> PISPIETVPVKLKPGMDGPKVKQWPLTEEKIKALVEICTEMEKEGKISKIGPENPYNTPVFAIKKKDSTKWRKLVDFRELNKRTQD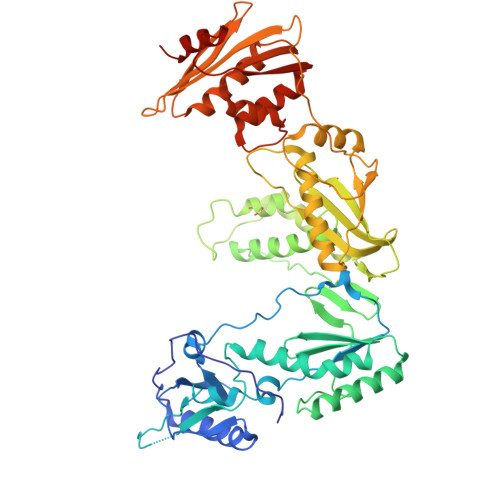FWEVQLGIPHPAGLKKKKSVTILDVGDAYFSVPLDEDFRKYTAFTIPSINNETPGIRYQYNVLPQGWKGSPAIFQSSMTKILEPFRKQNPDIVIYQYMDDLYVGSDLEIGQHRTKIEELRQHLLRWGLTTPDKKHQKEPPFLWMGYELHPDKWTVQPIVLPEKDSWTVNDIQKLVGKLNWASQIYPGIKVRQLCKLLRGTKALTEVIPLTEEAELELAENREILKEPVHGVYYDPSKDLIAEIQKQGQGQWTYQIYQEPFKNLKTGKYARMRGAHTNDVKQLTEAVQKITTESIVIWGKTPKFKLPIQKETWETWWTEYWQATWIPEWEFVNTPPLVKLWYQLEKEPIVGAETFYVDGAANRETKLGKAGYVTNRGRQKVVTLTDTTNQKTELQAIYLALQDSGLEVNIVTDSQYALGIIQAQPDQSESELVNQIIEQLIKKEKVYLAWVPAHKGIGGNEQVDKLVSAGIRKVL> TSKFPHLTFES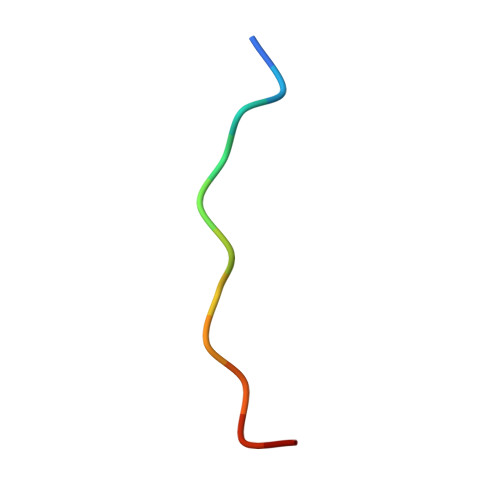P P-type ATPases, including ATP7A and ATP7B, are responsible for active copper efflux that is essential for maintaining copper homeostasis in mammalian cells. These two proteins are also known as Menkes (MNK) and Wilson (WLN) disease proteins, since dysfunction of ATP7A and ATP7B leads to these diseases, respectively. ATPases contain six metal-binding domains (MBDs) that share high sequence homology with Atox1, a chaperone delivering copper to ATPase, and exhibit similar copper-binding properties. In summary, tetrathiomolybdate (TM) can react with the metal-binding domain of ATPases (WLN4) and form a Mo2S6O2-centered protein dimer.

Since copper was not observed in the crystal structure of the TM-WLN4 complex, this indicates that the reaction with TM expelled copper ions from Cu-WLN4, suggesting the dimerization of WLN4 does not require copper ions. To verify this assumption, we reacted apo-WLN4 with TM, and tested whether TM can react with apo-WLN4 to generate the same protein dimer. SEC-MALS analysis showed that incubation of apo-WLN4 with TM generated a product with a molecular weight of 15 kDa, indicating that reaction of apo-WLN4 also results in a protein dimer. To further confirm the assumption that copper ions are not needed for the TM-mediated dimerization of WLN4, we incubated apo-WLN4 with TM and solved the crystal structure of the TM-WLN4 complex. Structural comparison showed that the overall dimeric structure of TM-WLN4 obtained from apo-WLN4 is identical to that from Cu-WLN4. The Fo – Fc maps of the Mo2S2O2 center also exhibit the same density features in both structures. These results further indicate that copper ions are not required for TM-mediated dimerization of WLN4. The reaction of apo-WLN4 with TM generated an identical structure to that of Cu-WLN4. These results indicate that formation of the copper-free Mo2S6O2 core plays a pivotal role in the formation of the dimeric TM-WLN4 adduct, which is rather different from the reaction of the copper chaperone Atx1 that generates a copper-linked TM-Cu-Atx1 ternary adduct. In addition, this Mo-centered copper-free adduct could be more relevant in the case of WLN since ATPases in the cytoplasm exist in apo-form, and copper-bound ATPases are localized at the cell membrane.

>[2x]TCSTTLIAIAGMTCASCVHSIEGMISQLEGVQQISVSLAEGTATVLYNPAVISPEELRAAIEDMGFEASVVS>MSKPIEIEIRRAPVLGSSMAYRETGAQDAPVVLFLHGNPTSSHIWRNILPLVSPVAHCIAPDLIGF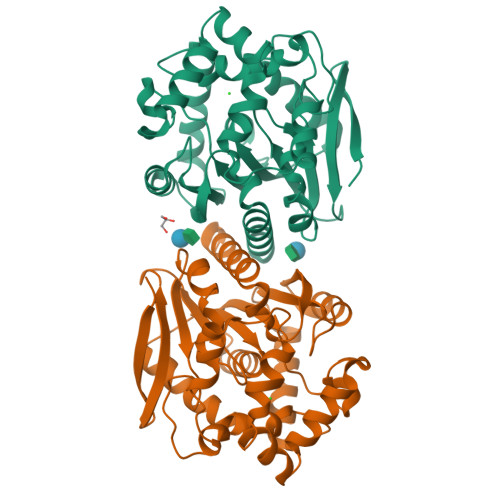GQSGKPDIAYRFFDHVRYLDAFIEQRGVTSAYLVAQDWGTALAFHLAARRPDFVRGLAFMEFIRPMPTWQDFHQDHAEAARAVFRKFRTPGEGEAMILEANAFVERVLPGGIVRKLGDEEMAPYRTPFPTPESRRPVLAFPRELPIAGEPADVYEALQSAHAALAASSYPKLLFTGEPGALVSPEFAERFAASLTRCALIRLGAGLHYLQEDHADAIGRSVAGWIAGIEAVRPQLAAHHHHHH[2x]Astroviruses are nonenveloped, positive-sense, single-stranded RNA viruses that belong to the Astroviridae family and are named after their ‘star-like’ appearance when observed by electron microscopy (EM). ORF1a and 1b encode non-structural polyproteins, while ORF2 encodes the viral capsid structural protein that is the target for host antibodies. The capsid core domain forms the icosahedral shell around the virus genome, whereas the capsid spike domain is thought to be responsible for the attachment and entry of the virus. The capsid spike domain is the primary target of serum antibodies, is the target of all known neutralizing monoclonal antibodies, and is being evaluated as a subunit vaccine antigen.

Porcine astrovirus 4 (PoAstV4) has been recently associated with respiratory disease in pigs. Therefore, we could not determine the spike domain boundaries based on sequence alignment alone, and instead determined the spike domain boundaries by predicting the structure of the full PoAstV4 capsid protein using AlphaFold2. We then designed a PoAstV4 spike construct containing residues 420 to 655 from the full-length capsid protein of PoAstV4. Size exclusion chromatography showed purified PoAstV4 spike protein eluted at the approximate size of a homodimer, which suggests that the recombinant protein is folded correctly. To further substantiate the folding of the recombinant PoAstV4 spike, we used X-ray crystallography to determine the structure of the PoAstV4 spike to 1.85 Å resolution. A trimmed AlphaFold2 model was used for molecular replacement. Structural alignment of the crystal structure of the PoAstV4 spike dimer with an AlphaFold2 predicted model using TM-align reveals an RMSD of 0.72 Å and a TM alignment score of 0.886, whereas an alignment with an AlphaFold3 predicted model reveals an RMSD of 0.49 Å and a TM alignment score of 0.992, demonstrating the accuracy of these structure prediction programs and improvements from AlphaFold2 to AlphaFold3. The PoAstV4 capsid spike crystal structure reveals a homodimeric protein formed of mainly beta-strands, similar to other animal and human astrovirus capsid spikes, and consistent with in-solution studies with size-exclusion chromatography. Interface analysis using the PDBePISA server reveals 4660 Å buried at the dimer interface, with 64–65 interacting residues in each chain. Compared to other experimentally solved astrovirus spike structures, the PoAstV4 spike has the highest structural similarity to murine astrovirus (MuAstV), as seen visually with a notable beta sheet cleft at the top of both spikes and by their high TM alignment score of 0.809.

>[4x]MGGPTTDPVQIYSPSLFGEPALYGSTATIGQRVPVAAVCMQAVGGAQKVYTYSLRELLDPVFVQNGNIIDITVIDLPTYPIYQKDGSDYSPIGDVYAAHFTTIGSSRPVQWTTVLWRANISKQIRLRGHATPTDQFLFFNPQLSMSGSNLPTTTYGLTVSSLVSLTERQEEINAGKWYLSTFVAFNGRREFDNYGIPFYLSLQQIDTQQGNYEPTTEAYNVGAMLNTATPLKLHLNAAAAELALVPR> M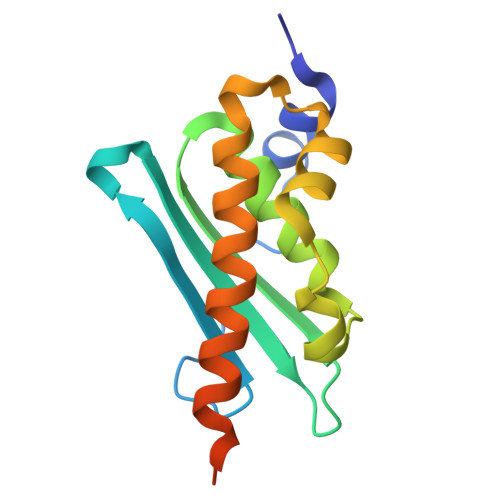ALSTQVVDHYENPRNVGSLDKTSKNVGTGLVGAPACGDVMKLQIQVDEKGKIVDARFKTFGCGSAIASSSLATEWVKGKTVEEALTIKNTDIAKELCLPPVKLHCSMLAEDAIKAALADYKLKQEPKKGEAEKKLEHHHHHH>[2x]MGRGSHHHHHHGMAMVQTKEIALEQLALTLTGDASWSSGPIYVVCDVG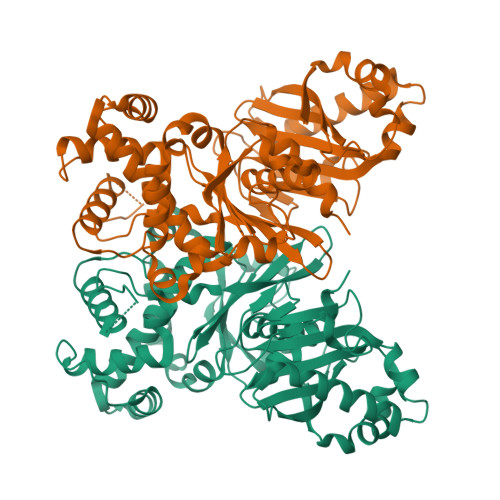GTSARVGFSQASQHDRSGLHIIYVRFKVTKSDIRQLLEFFDEVLQHLKKNLPDHGASFLRRVASGAVSVPGPVTNGQLAGPFNNLKGIARLVDYPVELFPKGRSALLNDLEAGAYGVLALSNAGILSDYFKVMWKGTQWDALSEGKPAGSTIGRGRCMVVAPGTGVGSSLIHYVGVSDSYIVLALECGSLSMSWCANEDSKYVQALAGYMASKAHAKGLDSTVAPIWEAASNGAGLEFNYAYAKEGQKASAPLKSAPEVAKLAKSGSDTAAIAAVDRLYKNLIGLTAETTMQFLPLTCVLMGDNVVANSFYFEKPENVKRLQARLHEHAMERQFKFLSRTTFLRQVSSVNINLLGCLGFGSQLS> MGNNTDDSAR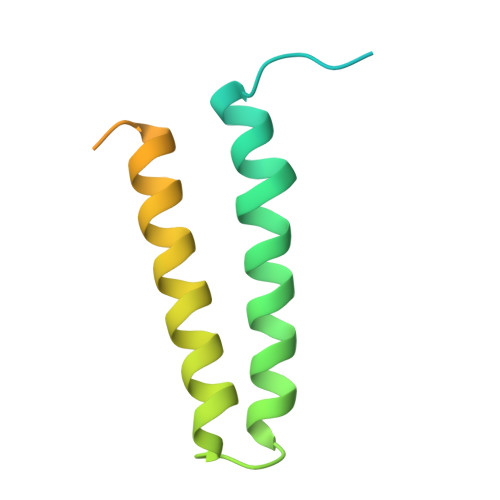NPFGFYTPPRVKEIGEPDVTDATLGSVYSEIISPVKDCILTVAKAVSFNPGGKDNTDAVEVLTELNTKVERAALNQPILTTKTERMFGAAESEKSSEPPSHDERGFKLSS alpha-L-psicofuranose | C6 H12 O6 | 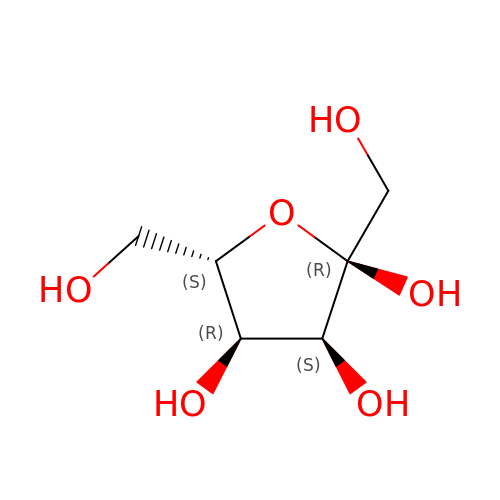RFSUNEUAIZKAJO-OMMKOOBNSA-N> MAESTQHKLDRIRPPRVQITYDVETGNAIEKKELPLVVGILADLSGKPEKPLPKLMERRFVEINRDNFN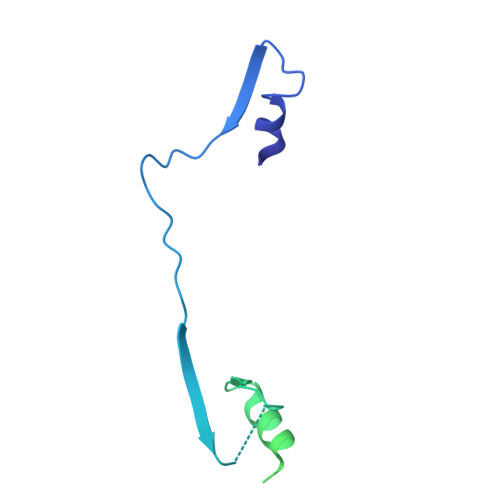DVLASIAPRAALQVDNTLSQDGSKLNIELHFDHIDDFDPVNIVRQVTPLRRLFEARQRLRDLLTKLDGNDDLDKLLQDVVANTEGLQEIRSARPQAENPAGAPGAEPAADEPAAEPQA>GANAMGVLISAVGDTDPFRNFHDGALIHIARKYRPEKVILIFSEHTAKKQGNIEKALFSIAPNYEPELIIHDPIISDNEVHIFDVMFQRFSDILQEYYTKEDEFILNLSSATPQIKSALFVINRLNGINVKAVQVSSPEHASNENIGHDNDENIDELIEVNKDNKVNFIDRTIEDNAEKFSQALLKKTARDFIEKFDYKAALDILDQLSDFPNLKSVREEIRDVVNCLSKQDVPKGLRHKKLKEEEQKILSAYLTIELQRER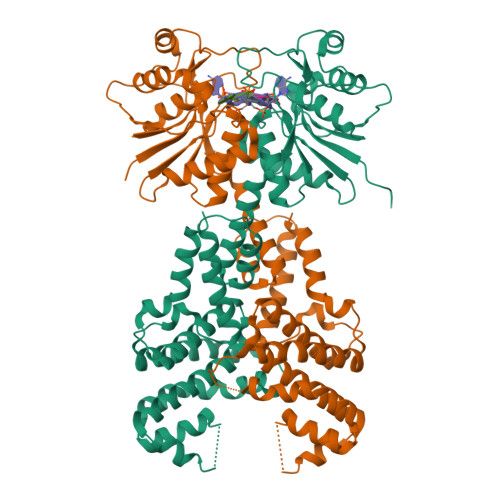GNVSESFIRIKNLTEFILEDYIKKRYPGLIDEYCEDIQKYYLSLFDYSKLLKATKEFKLKRTIAPIIDMNSSRNKVAHSLSPLDSDAVKQLGIAMKTLKTLVREQYHFSQSDFNFYQDLNKILLTKLN[2x]> XXXXXXXXXXXXLPAIAVIGDQSSGKSSVLEALSGVALPRGSGIVTRCPLVLKLKKLVNEDKWRGKVSYQDYEIEISDASEVEKEINKAQNAIAGEGMGISHELITLEISSRDVPDLTLIDLPGITRVAVGNQPADIGYKIKTLIKKYIQRQETISLVVVPSNVDIATTEALSMAQEVDPEGDRTIGILTKPDLVDKGTEDKVVDVVRNLVFHLKKGYMIVKCRGQQEIQDQLSLSEALQREKIFFENHPYFRDLLEEGKATVPSLAEKLTSELITHISKSLPLLXXXXXXXXXXXXXXXXXX;> SQYEEKVRPCIDLIDSLRALGVEQDLALPAIAVIGDQSSGKSSVLEALSGVALPRGSGIVTRCPLVLKLKKLVNEDKWRGKVSYQDYEIEISDASEVEKEINKAQNAIAGEGMGISHELITLEISSRDVPDLTLIDLPGITRVAVGNQPADIGYKIKTLIKKYIQRQETISLVVVPSNVDIATTEALSMAQEVDPEGDRTIGILTKPD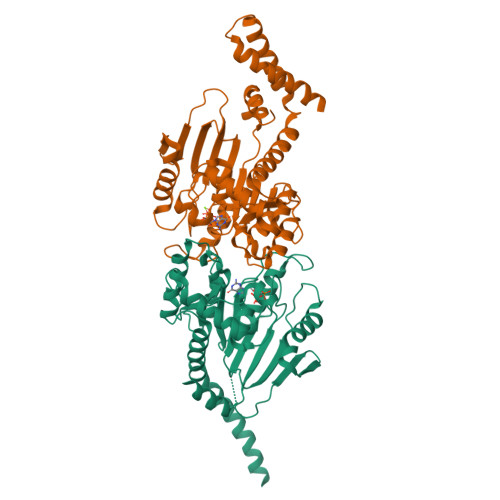LVDKGTEDKVVDVVRNLVFHLKKGYMIVKCRGQQEIQDQLSLSEALQREKIFFENHPYFRDLLEEGKATVPSLAEKLTSELITHISKSLPLLENQIKETHQRITEELQKYGGDPKAKFLKERLARLTQARRRLAQFPG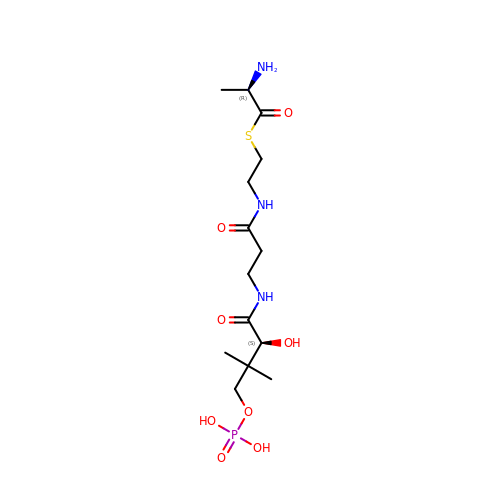S-[2-[3-[[(2S)-3,3-dimethyl-2-oxidanyl-4-phosphonooxy-butanoyl]amino]propanoylamino]ethyl] (2R)-2-azanylpropanethioate | C14 H28 N3 O8 P S | YOANCVNRLJJRIX-MWLCHTKSSA-N>[6x]HPSSPPVVDTVHGKVLGKFVSLEGFAQPVAIFLGIPFAKPPLGPLRFTPPQPAEPWSFVKNATSYPPMCTQDPKAGQLLSELFTNRKEN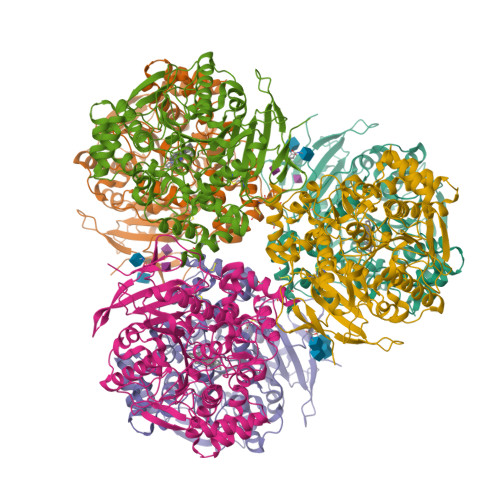IPLKLSEDCLYLNIYTPADLTKKNRLPVMVWIHGGGLMVGAASTYDGLALAAHENVVVVTIQYRLGIWGFFSTGDEHSRGNWGHLDQVAALRWVQDNIASFGGNPGSVTIFGESAGGESVSVLVLSPLAKNLFHRAISESGVALTSVLVKKGDVKPLAEQIAITAGCKTTTSAVMVHCLRQKTEEELLETTLKMKFLSLDLQGDPRESQPLLGTVIDGMLLLKTPEELQAERNFHTVPYMVGINKQEFGWLIPMLMSYPLSEGQLDQKTAMSLLWKSYPLVCIAKELIPEATEKYLGGTDDTVKKKDLFLDLIADVMFGVPSVIVARNHRDAGAPTYMYEFQYRPSFSSDMKPKTVIGDHGDELFSVFGAPFLKEGASEEEIRLSKMVMKFWANFARNGNPNGEGLPHWPEYNQKEGYLQIGANTQAAQKLKDKEVAFWTNLFAKKAVEKPPQTEHIEL>[5x]MALRSAQGDGPTSGHWDGGAEKADFNAKRKKKVAEIHQALNSDPTDVAALRRMAISEGGLLTDEIRRKVWPKLLNVNANDPPPISGKNLRQMSKDYQQVLLDVRRSLRRFPPGMPEEQREGLQEELIDIILLILERNPQLHYYQGYHDIVVTFLLVVGERLATSLVEKLSTHHLRDFMDPTMDNTKHILNYLMPIIDQVNPELHDFMQSAEV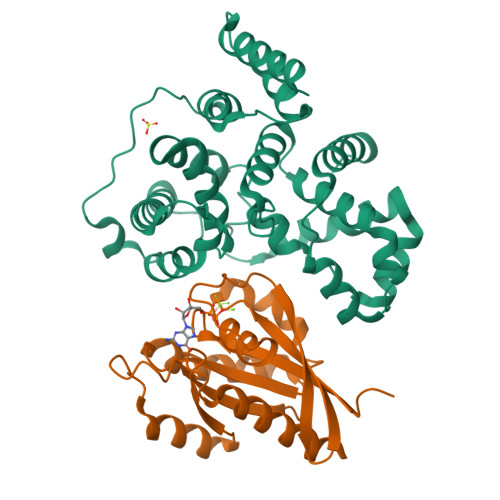GTIFALSWLITWFGHVLSDFRHVVRLYDFFLACHPLMPIYFAAVIVLYREQEVLDCDCDMASVHHLLSQIPQDLPYETLISRAGDLFVQFPPS;>GHMPEYDYLFKLLLIGDSGVGKSCLLLRFADDTYTESYISTIGVDFKIRTIELDGKTIKLQIWDTAGQERFRTITSSYYRGAHGIIVVYDVTDQESYANVKQWLQEIDRYASENVNKLLVGNKSDLTTKKVVDNTTAKEFADSLGIPFLETSAKNATNVEQAFMTMAAEIKKRMG[5x]> MNDTLLNAYSGIKTHQFGIDSLSNNIANVNTLGYRSNDPEFKTLFSSHLDALNAKSVVTNDRNYGVTGSGNVLSNKDGEYMPSEGEFHMAYQGKGWFVIGPNKNGEMTINKDGFSKKQDNFLTRAGNFARDADGYLVTPEGYYVYGIDLKKIKDGTLNSTARDEDIEKLHGNTLSPLQIPQDLTYQPVLSTKVGISVNLNPKDHLKGVQDFFLNDKGEIIKERFLNQDINALANDDNEPIDAITNRKLNVSIQKENGKKEDFVFTYGDAEKGENQFKTLGDLQKLLKEKTGLDLNLIKSEKDAKSPPLLLEIANPSQTPITFSLSGGIADKLGLNANGMELKKGISRDSVAIKIPYYSTEVDIYDKAGDKYLLQSEYYMTNSNDPTSSPTSKRKNQTWEVKSYIVDPKNKTPINDPTWEIVGFDSATHKMKSAPMTLDFKGNKLTYSLDKSENHDSSDLSYQDSKLLEASQDGKPRGIFRDMRIEENGVISLAFSNGVVEPVARIGILAFTNDQGLRKIGGNLYEMQEGTINGENRPLSGNPILGWDEEGKLKFGKIRHKYLETSNVNAGNALTNLILMQRGYSMNARAFGAGDDMIKEAISLKK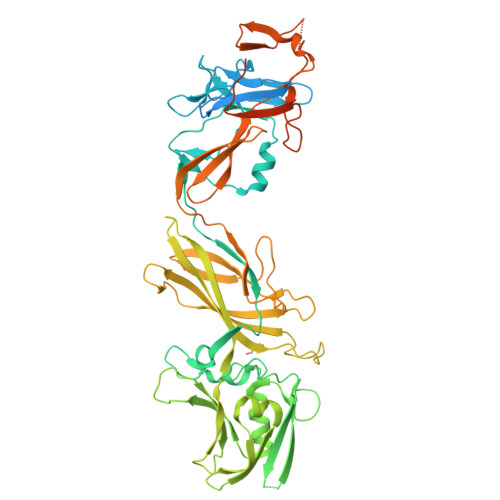ENLYFQSHHHHHH>[2x]MQDEVVLLDFWPSPFGMRVRIA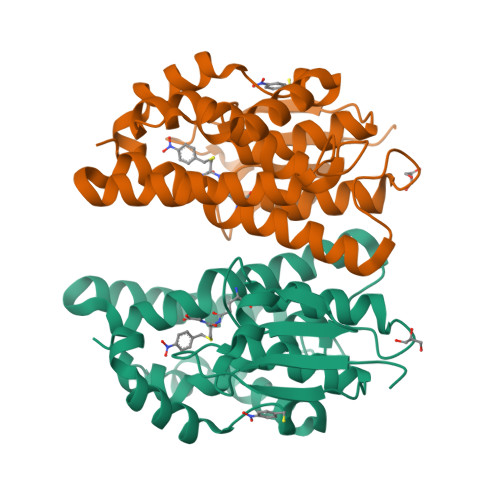LAEKGIKYEYKEEDLRNKSPLLLQMNPVHKKIPVLIHNGKPICESLIAVQYIEEVWNDRNPLLPSDPYQRAQTRFWADYVDKKIYDLGRKIWTSKGEEKEAAKKEFIEALKLLEEQLGDKTYFGGDNLGFVDIALVPFYTWFKAYETFGTLNIESECPKFIAWAKRCLQKESVAKSLPDQQKVYEFIMDLRKKLGIE> AMLPPDILQNGEFETIYFQTNPTYIKSPIHIPKSTIGKPDTVKIRHFFALLHQDLVVLGLEVFVYLQIYSDFVEKYVYVSKCDTVGLEKSTIKIGKVIGPVLQYIINYNGYKIKMKNLDEKSKDLSDPSTLVRLQRLRDKLPDIYPNLPYYNDIPPKEECIEYRTLPKTQNLRLCVFTKPAKEALFPNSAKNPYKNLLNGQSLLRWWISIIDSITKGWNNHKLMIPGADKYATRKFIEKYSDWSEGHIFKKDGLAVQAIPLFPDDPKGRFLELVIVECRYGKMTVSRFYQELAYRQEFLLGDCVSLIGCCKENLEVTYHDDLVSTVTISEYKEFMNLLKLVDF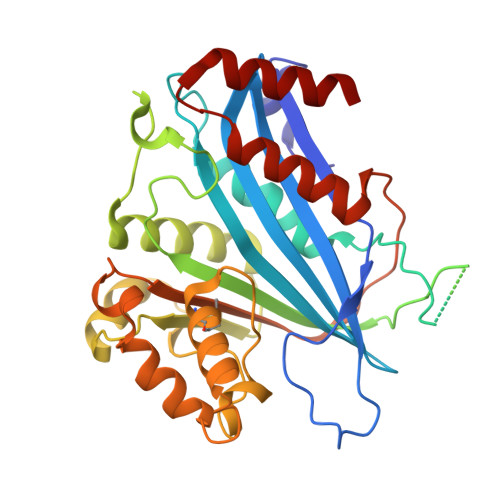SDRVEVSNFVSNYRKSK> ASPSSELRRALEANEFIPYYQPLSPGQGGRWIGVEVLMRWRHPREGLIRPDLFIPFAERSGLIVPMTRALMRQVAEDLGGHAGKLEPGFHIGFNISATHCHELALVDDCRELLAAFPPGHITLVLELTERELIESSEVTDRLFDELHALGVKIAIDDFGTGHSSLAYLRKFQVD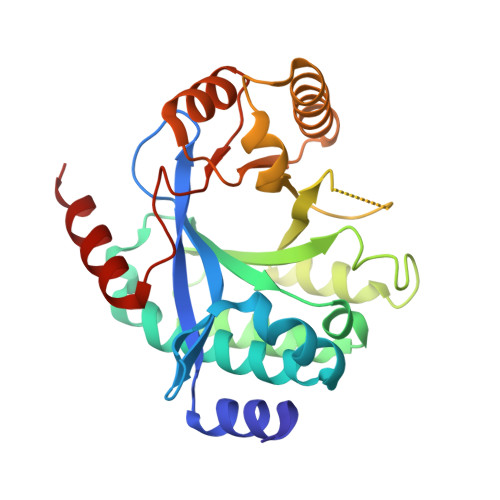CLKIDQSFVARIGIDTLSGHILDSIVELSAKLDLDIVAEGVETPEQRDYLAARGVDYLQGYLIGRPMPLESLLSSLTVQEGQ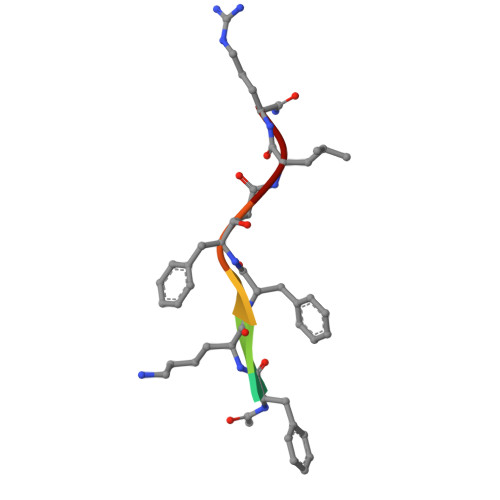> XFKFFLR> MSDIRHSLLRRDALSAAKEVLYHLDIYFSSQLQSAPLPIVDKGPVELLEEFVFQVPKERSAQPKRLNSLQELQLLEIMCNYFQEQTKDSVRQIIFSSLFSPQGNKADDSRMSLLGKLVSMAVAVCRIPVLECAASWLQRTPVVYCVRLAKALVDDYCCLVPGSIQTLKQIFSASPRFCCQFITS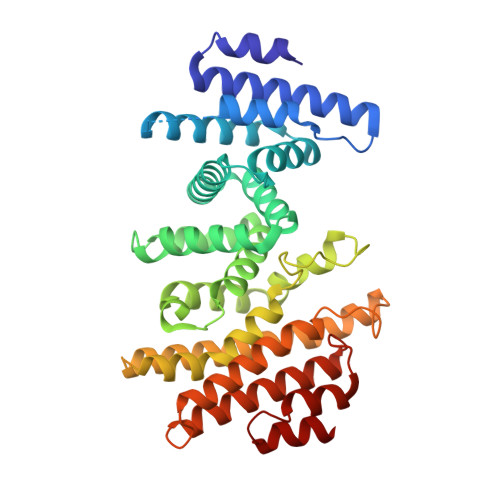VTALYDLSSDDLIPPMDLLEMIVTWIFEDPRLILITFLNTPIAANLPIGFLELTPLVGLIRWCVKAPLAYKRKKKPPLSNGHVSNKVTKDPGVGMDRDSHLLYSKLHLSVLQVLMTLQLHLTEKNLYGRLGLILFDHMVPLVEEINRLADELNPLNASQEIELSLDRLAQALQVAMASGALLCTRDDLRTLCSRLPHNNLLQLVISG[(6-oxo-4-phenyl-1,6-dihydropyrimidin-2-yl)sulfanyl]acetonitrile 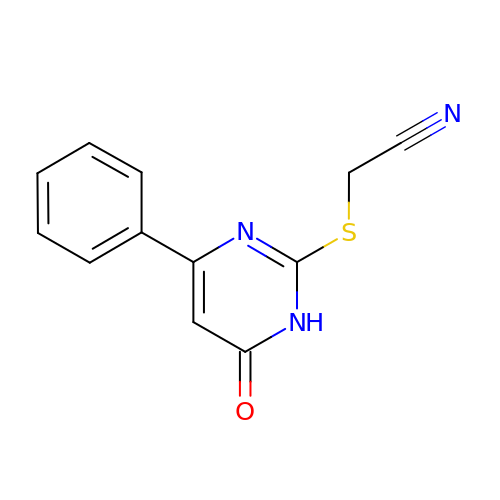| C12 H9 N3 O S | LOXMFYYAURQRNF-UHFFFAOYSA-N> GAMGFGDLKSPAGLQVLNDYLADKSYIEGYVPSQADVAVFEAVSSPPPADLCHALRWYNHI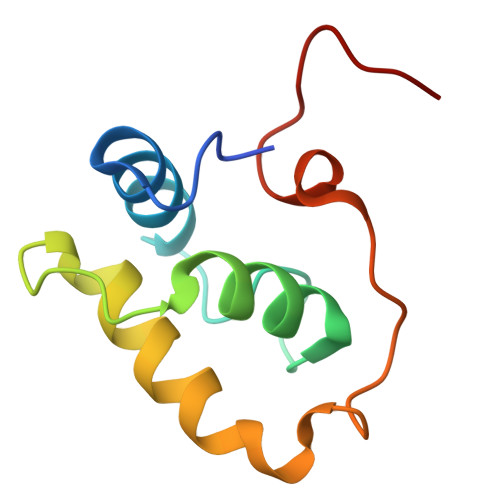KSYEKEKASLPGVKKALGKYGPADVEDTT> ALSAKLTLDKVDLKGKRVIMRVDFNVPMKNNQITNNQRIKAAIPSIKHCLDNGAKSVVLMSHLGRPDGIPMPDKYSLEPVADELKSLLNKDVIFLKDCVGPEVEQACANPDNGSIILLENLRFHVEEEGKGKDSSGKKISADPAKVEAFRASLSKLGDVYVNDAFGTAHRAHSSMVGVNLPQKASGFLMKKELDYFSKALEKPERPFLAILGGAKVKDKIQLIKNMLDKVNFMIIGGGMAYTFLKELKNMQIGASLFDEEGATIVKEIMEKAEKNGVKIVFPVDFVTGDKFDENAKVGQATIESGIPSGWMGLDCGPESIKINAQIVAQAKLIVWNGPIGVFEWDAFAKGTKALMDEVVKATSNGCVTIIGGGDTATCCAKWGTEDKVSHVSTGGGASLELLEGKILPG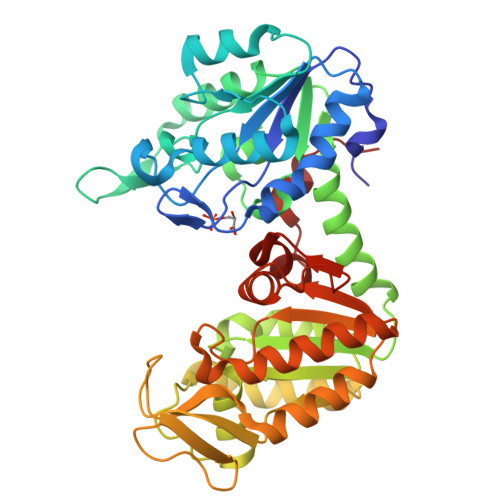VEALSNM> SQTIDKINSCYPLFEQDEYQELFRNKRQLEEAHDAQRVQEVFAWTTTAEYEALNFRREALTVDPAKACQPLGAVLCSLGFANTLPYVHGSQGCVAYFRTYFNRHFKEPIACVSDSMTEDAAVFGGNNNMNLGLQNASALYKPEIIAVSTTCMAEVIGDDLQAFIANAKKDGFVDSSIAVPHAHTPSFIGSHVTGWDNMFEGFAKTFTADYQGQPGKLPKLNLVTGFETYLG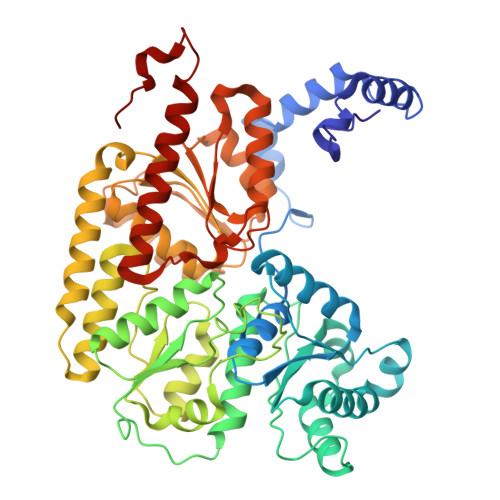NFRVLKRMMEQMAVPCSLLSDPSEVLDTPADGHYRMYSGGTTQQEMKEAPDAIDTLLLQPWQLLKSKKVVQEMWNQPATEVAIPLGLAATDELLMTVSQLSGKPIADALTLERGRLVDMMLDSHTWLHGKKFGLYGDPDFVMGLTRFLLELGCEPTVILSHNANKRWQKAMNKMLDASPYGRDSEVFINCDLWHFRSLMFTRQPDFMIGNSYGKFIQRDTLAKGKAFEVPLIRLGFPLFDRHHLHRQTTWGYEGAMNIVTTLVNAVLEKLDSDTSQLGKTDYSFDLVR> GANSLSVHQLAAQGEMLYLATRIEQENVINHTDEEGFTPLMWAAAHGQIAVVEFLLQNGADPQLLGKGRESALSLACSKGYTDIVKMLLDCGVDVNEYDWNGGTPLLYAVHGNHVKCVKMLLESGADPTIETDSGYNSMDLAVALGYRSVQQV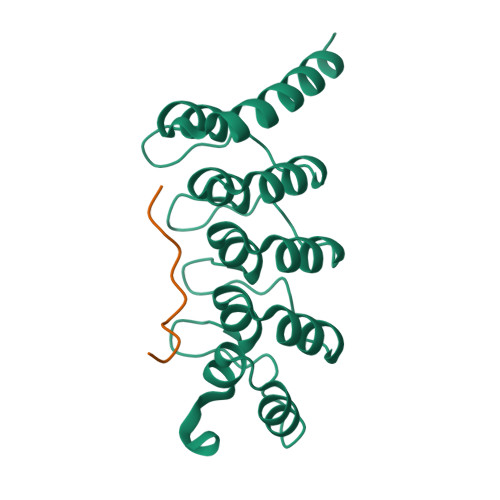IESHLLKLLQNIKE;> LLPTLPKLPSL> MSSTILVIHGPNLNLLGKREPEVYGHLTLDNINRQLIAQAEQASITLDTFQSNWEGAIVDRIHQAQTEGVKLIIIN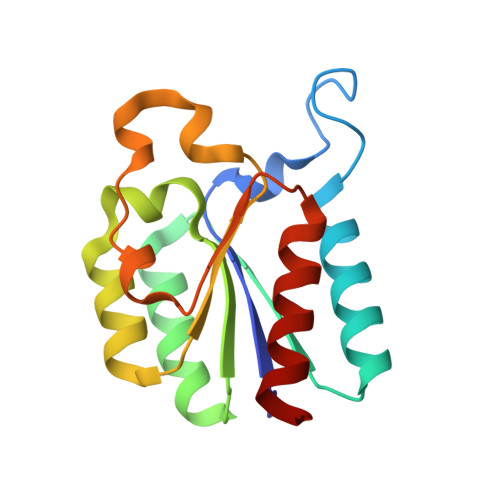PAALTHTSVALRDALLGVAIPFIEVHLSNVHAREAFRHHSYLSDKAIGVICGLGAKGYSFALDYAIEKIQP> 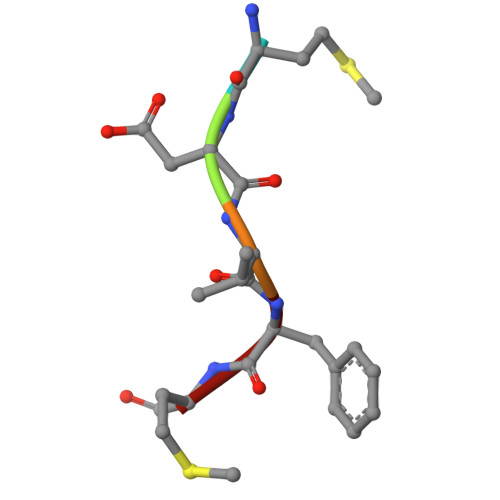MDVFM> GPGSAENEK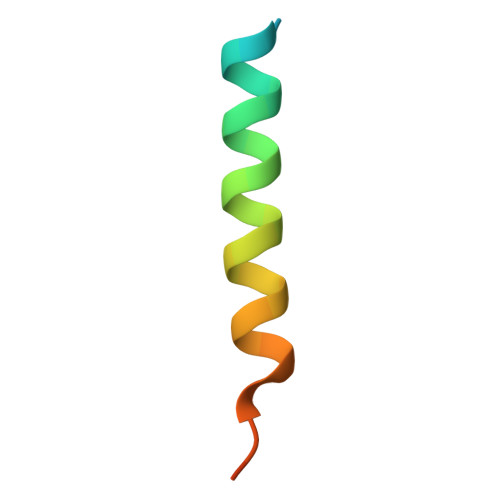DSRRRQARLQKELAEAAKEPLPVEQ> MAHHHHHHMITERELLDYIVNNGGFLDIEHFSKVYGVEKQEVVKLLEALKNKGLIAV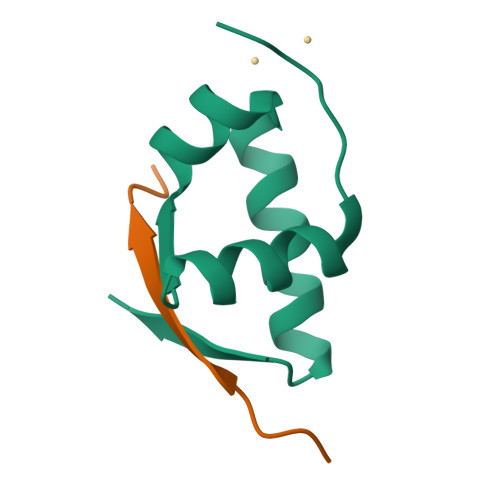ES;> SEIPLPIPVKVINTL Streptococcus pneumoniae scavenges essential zinc ions from the host during colonization and infection. This is achieved by the ATP-binding cassette transporter, AdcCB, and two solute-binding proteins (SBPs), AdcA and AdcAII. AdcAII belongs to the cluster A-I subgroup of SBPs, consisting of a conserved structural fold of two (β/α)4 domains connected by a rigid α-helix, with the metal-binding site located at the interface between the N- and C-terminal lobes (Loisel et al., 2008; Yukl, 2017).

In this study, we investigated the Zn(II)-binding mechanism of AdcAII by mutating each of the four Zn(II)-coordinating residues in the SBP. Structural analyses of Zn(II)-bound AdcAII variants revealed that specific regions within the protein underwent conformational changes via direct coupling to each of the metal-binding residues. The binding site mutations impacted protein conformation and interaction with Zn(II) to differing extents. Quantitative in vitro metal-binding assays combined with affinity determination and phenotypic growth assays revealed that each of the four Zn(II)-coordinating residues contributes to metal binding by AdcAII. Intriguingly, the phenotypic growth impact of the mutant adcAII alleles was, in general, independent of affinity, suggesting that the Zn(II)-bound conformation of the SBP is crucial for efficacious metal uptake. Taken together, these data demonstrate the importance of SBP-metal complex conformation for bacterial Zn(II) uptake.

> HMGTGSLGGGFPGKGMKIVTSFYPIYAMVKEVSGDLNDVRMIQSSSGIHSFEPSANDIAAIYDADVFVYHSHTLESWAGSLDPNLKKSKVKVLEASEGMTLERVPGLEDVEAGDGVDEKTLYDPHTWLDPEKAGEEAQIIADKLSEVDSEHKETYQKNAQAFIKKAQELTKKFQPKFEKATQKTFVTQHTAFSYLAKRFGLNQLGIAGISPEQEPSPRQLTEIQEFVKTYKVKTIFTESNASSKVAETLVKSTGVGLKTLNPLQSDPQNDKTYLENLEENMSILAEELKGNLYFQ2-azanylidene-N-(4-methylphenyl)-8-oxidanyl-chromene-3-carboxamide | C17 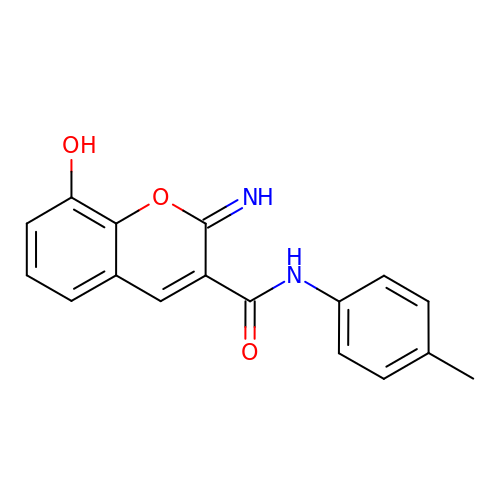H14 N2 O3 | SKZQOFVKMNLPBF-VLGSPTGOSA-N> MAPKAVLVGLPGSGKSTIGRRLAKALGVGLLDTDVAIEQRTGRSIADIFATDGEQEFRRIEEDVVRAALADHDGVLSLGGGAVTSPGVRAALAGHTVVYLEI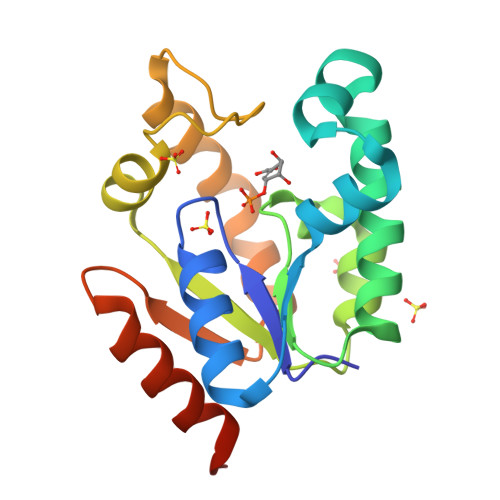SAAEGVRRTGGNTVRPLLAGPDRAEKYRALMAKRAPLYRRVATMRVDTNRRNPGAVVRHILSRLQVPSPSEAAT> LSKFGGECSLKHNTC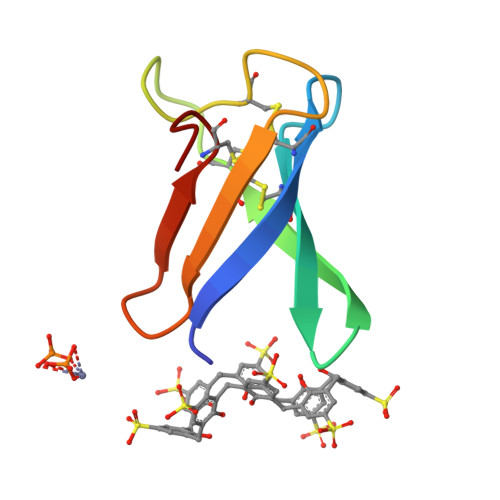TYLKGGKNHVVNCGSAANKKCKSDRHHCEYDEHHKRVDCQTPV> MGAKPKAQTVGWRYYFDIHFALGKKVDEVCAIRASGKTAWKGSITSNGQVRINAPELFGGDKGEGGLDGTLDVLFGEEDQGVLPRLAAMLGGLVPAFRGVTTCFYSGLVTSVNPYPKKWEILRRGGNRLWDGNPWYPEKQFVWLADGQIKAMNPAHILYLVYTGRDFRGLARTRMDEASWRAAADTLYAEGFGLCFEWTRSDSFKNFCETVKSHIGAEVYPNRQ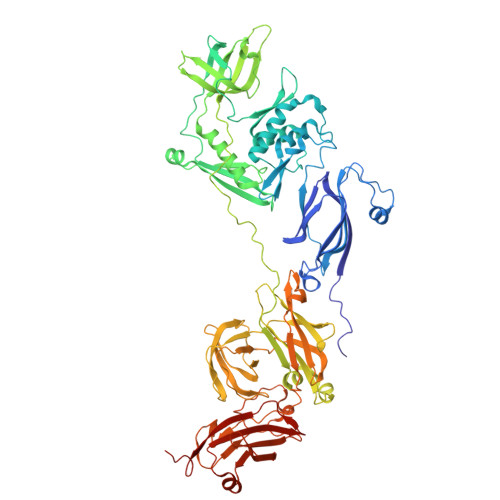TGQISIRLLRDDYNVADLPLFDEDSGLLEITQEKTGSTSLAPSQLIVKYIDQIDGAQRQIIVNNNAVAASQGRRSSEEIEFLGVPTGELAGRVGEREMRLKTTGLKRYKGVFDRRARSLNPGQPFLIRSTPRGIPETVVRVGRIEDNFLGDGKITLTVVQDQFNLPATTGVAPPPPGWTPPDRTPRAITVRRLIEAPYRELAGVIDPANLQLLDVSASYLAALAEAPTSLSQSYTLTDRVGSSGAFVDRGTGDWCPTGLLAAELPLAAGPNVVTLTNATRLEDVTVGQAAVVDDEIVRVDAVNYASGTVTLARGCADTVPAKHLAGARVWFYDTFEAVDETVYSQGVTLQARLLTNTSEGQLAPALAATDSLTLTGRQGKPYPPGQFRINGSAYPTKVYGALSVSWAKRDRIGQADQLIDTTVGNIGPEDGATVTLQVYSGTTLKRTYAGLTSSSWSYPLAEDMADGPLQDVRLVLRSVRDGIDSWQQHDITIERHGLGFRLGEELGGVSA> SKVCIIAWV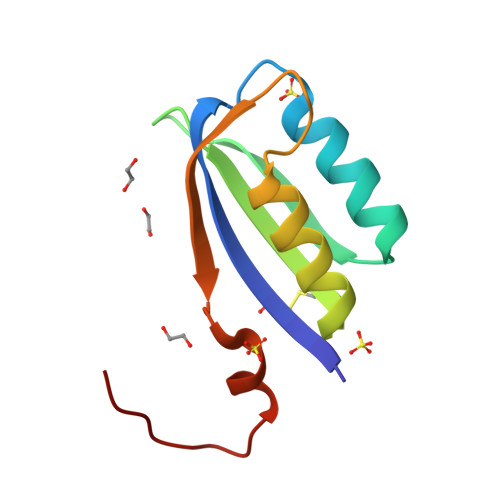YGRVQGVGFRYTTQYEAKRLGLTGYAKNLDDGSVEVVACGEEGQVEKLMQWLKSGGPRSARVERVLSEPHHPSGELTDFRIRLE>MATLTAKNLAKAYKGRRVVEDVSLTVNSGEIVGLLGPNGAGKTTTFYMVVGIVPRDAGNIIIDDEDISLLPLHARARRGIGYLPQEASIFRRLSVFDNLMAVLQIRDDLTSEQRQDRANELMEEFHIEHLRDSLGQALSGGERRRVEIARALAANPKFILLDEPFAGVDPISVIDIKRIIEHLRDSGLGVLITDHNVRETLAVCERAYIVSQGNLIAHGTPQQILEDDHVKRVYLGEDFRL[4x];>MSKTRRWVIILLSLVALILIGVNLADRDDTQTEVINNNDPTYKSDHSDTVVYSPEGALNYRLIAQHVEYFSDDGISWFTQPVMTTFDKDKVPTWSIKSDRAKLTNDRMLYLYGHVEVNALTADSQLRKITTDNAQINLVTQDVTSQDLVTLYGTTFNSSGLRMRGNLRSKNAELIEKVRTSYEIQNKQTQPLVPR[2x];>[2x]MIIIRYLVRETLKSQLAILFILLLIFFCQKLVKILGAAVDGEIPTNLVLSLLGLGIPEMAQLILPLSLFLGLLMTLGKLYTESEITVMHACGLSKAVLVKAAMILALFTGIVAAVNVMWAGPMSSRHQDEVLAEAKANPGMAALAQGQFQQATDGNSVLFIESVDGSKFNDVFLAQLRTKGNARPSVVVADSGQLAQRKDGSQVVTLNKGTRFEGTAMLRDFRITDFQNYQAIIGHQAVALDPTDTEQMDMRTLWNTDTDRARAEFHWRITLVFTVFMMALIVVPLSVVNPRQGRVLSMLPAMLLYLIYFLLQTSIRSNGAKGKLDPMVWTWFVNSLYILLALGLNLWDTVPVRRIRARFSRKGAI;>[2x]MQAFGVLDRYIGKTIFTTIMMTLFMLVSLSGIIKFVDQLKKAGQGSYDALGAGMYTLLSVPKDVQIFFPMAALLGALLGLGMLAQRSELVVMQASGFTRLQVALSVMKTAIPLVLLTMAIGEWVAPQGEQMARNYRAQAMYGGSLLSTQQGLWAKDGQNFVYIERVKGDDELGGVSIYAFNDERRLQSVRHASSAKFDPEHKQWRLSQVDESDLTNPKQITGSQTVSGTWKTNLTPDKLGVVALDPDALSISGLHNYVKYLKSSGQDAGRYQLNMWSKIFQ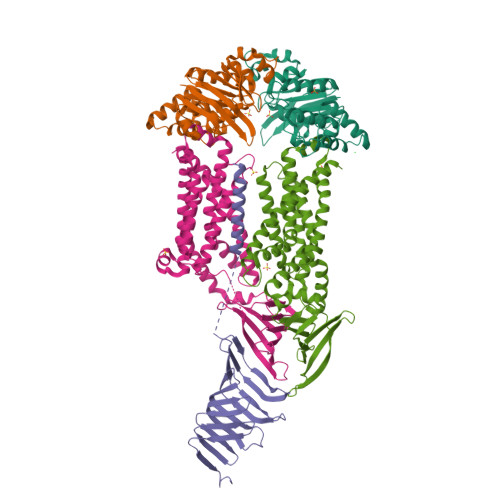PMSVAVMMLMALSFIFGPLRSVPMGVRVVTGISFGFVFYVLDQIFGPLTLVYGIPPIIGALLPSASFLLISLWLLLKRS> DITVYNGQH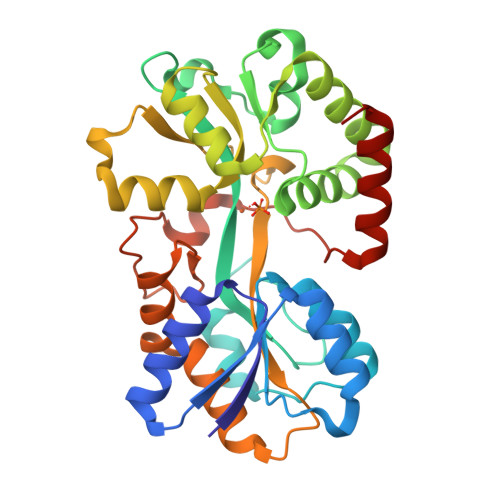KEAATAVAKAFEQETGIKVTLNSGKSEQLAGQLKEEGDKTPADVFYTEQTATFADLSEAGLLAPISEQTIQQTAQKGVPLAPKKDWIALSGRSRVVVYDHTKLSEKDMEKSVLDYATPKWKGKIGYVSTSGAFLEQVVALSKMKGDKVALNWLKGLKENGKLYAKNSVALQAVENGEVPAALINNAYWYNLAKEKGVENLKSRLYFVRHQDPGALVSYSGAAVLKASKNQAEAQKFVDFLASKKGQEALVAARAEYPLRADVVSPFNLEPYEKLEAPVVSATTAQDKEHAIKLIEEAGLK>[4x]MSLFDKKHLVSPADALPGRNTPMPVATLHAVNGHSMTNVPDGMEIAIFAMGAFWGVERLFWQLPGVYSTAAGYTGGYTPNPTYREVASGDTGHAEAVRIVYDPSVISYEQLLQVFWENHDPAQGMRQGNDHGTQYRSAIYPLTPEQDAAARASLERFQAAMLAADDDRHITTEIANATPFYYAEDDHQQYLHKNPYGYAGIGGIG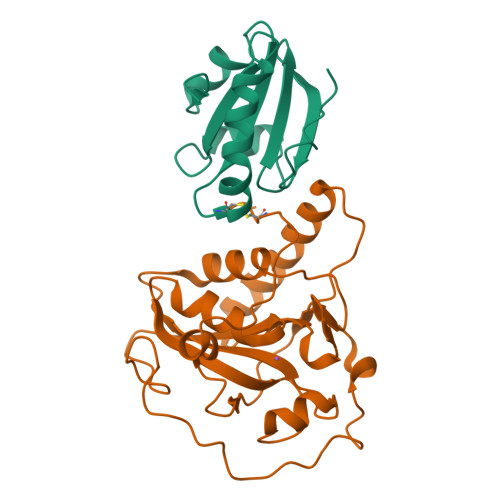VCLPPEA;>[3x]MSDKIIHLTDDSFDTDVLKADGAILVDFWAEWCGPSKMIAPILDEIADEYQGKLTVAKLNIDQNPGTAPKYGIRGIPTLLLFKNGEVAATKVGALSKGQLKEFLDANLA> MERRLIFGTIASKMSLAPEADLDSLIIRNDSLSGAVIAAIMQEAGLRAVRKNRYVILQSDLEEAY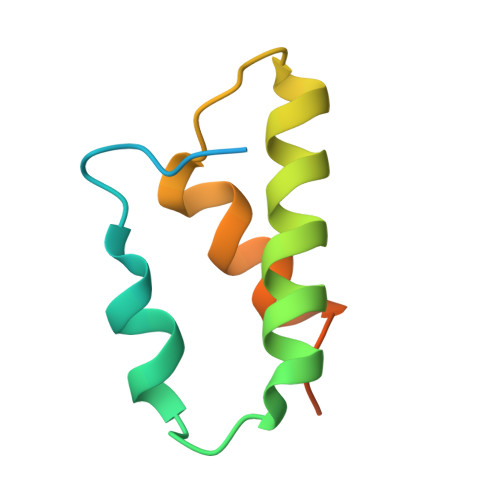ATQVKTDNTVDKFDFYK>MRTRSTLTDKNGITWYYEQEGSGPHVVLIPDGLGECHMMDKPMSMIAGMGFTCTTFDMPGFSRSWDAPPETYQDVTAQKLASYVISILDELHIDYATFWGCSSGGATVLALAADYPERMRNGLPHEVPTAAGPHFGQLLKLAEMEDEAIVKMLGEEMPKLGFGHDFTAWHELGEEAHARMRKNYPRWARGYPHTLPLSSPTGKEDLIKRPLDWTVGGDTPTRMFFDNIVT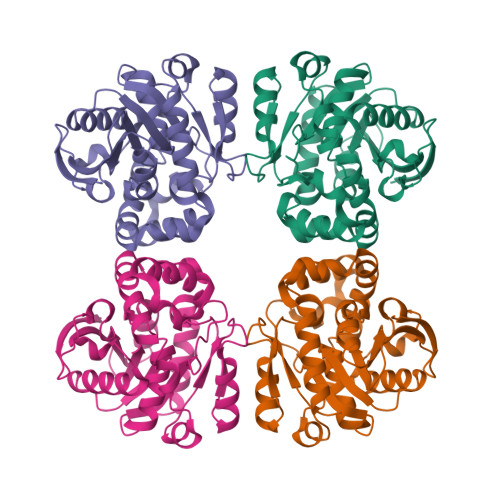ASKAGIPIATLPGMHFPYVSHPEVLVKHIVDTTRKYL[4x]Recent work has shown that the metal‐dependent protein phosphatase PPM1H counteracts LRRK2 by dephosphorylating Rabs. The crystal structure of PPM1H reveals a structurally conserved phosphatase fold that strikingly has evolved a 110‐residue flap domain adjacent to the active site. Cellular assays, crosslinking and 3‐D modelling suggest that the flap domain encodes the docking motif for phosphorylated Rabs. Therefore, PPM1H has acquired a Rab‐specific interaction domain within a conserved phosphatase fold.

Full‐length PPM1H expressed in E. coli cells was unstable and prone to degradation, thus difficult to crystallize. To design a crystallisable protein, the N‐terminal residues 1‐32 were eliminated due to predicted flexibility. We also introduced a D288A mutation (PPM1HDA) that destabilizes a third metal ion (Mg2+/Mn2+) at the active site. Previous studies of PPM1A (D146A) showed that this variant acts as a substrate‐trapping mutant (Debnath et al, 2018). Crystals were grown of PPM1HDA that diffracted to 3.1 Å resolution, but no crystals grew of the WT enzyme. The variants PPM1HDA, PPM1HWT‐LD, and PPM1HDA‐LD have identical 3‐D structures with two Mg2+ ions at the active site. However, all of the structures are identical with only minor differences arising from flexible loops and the presence or absence of the third metal ion at the active site. The asymmetric unit in all 4 structures is a dimer that is facilitated by interactions between α3 of the flap domains, as well as contacts between the flap domain (residues 356–360) and α2 of the catalytic domain.

>[2x]GSHMSDLPLRFPYGRPEFLGLSQDEVECSADHIARPILILKETRRLPWATGYAEVINAGKSTHNEDQASCEVLTVKKKAGAVTSTPNRNSSKRRSSLPNGEGLQLKENSESEGVSCHYWSLFDGHAGSGAAVVASRLLQHHITEQLQDIVDILKNSAVLPPTCLGEEPENTPANSRTLTRAASLRGGVGAPGSPSTPPTRFFTEKKIPHECLVIGALESAFKEMDLQIERERSSYNISGGCTALIVICLLGKLYVANAGASRAIIIRNGEIIPMSSEFTPETERQRLQYLAFMQPHLLGNEFTHLEFPRRVQRKELGKKMLYRDFNMTGWAYKTIEDEDLKFPLIYGEGKKARVMATIGVTRGLGDHDLKVHDSNIYIKPFLSSAPEVRIYDLSKYDHGSDDVLILATDGLWDVLSNEEVAEAITQFLPNCDPDDPHRYTLAAQDLVMRARGVLKDRGWRISNDRLGSGDDISVYVIPLIHGNKLS DyPs (dye-decolorizing peroxidases) (EC 1.11.1.19) represent a new family of haem peroxidases widespread in bacteria, archaea, fungi and other micro-organisms. In the present study, we expressed A. auricula-judae DyP in E. coli, solved the crystal structure of the recombinant enzyme and several site-directed variants, and used PELE (Protein Energy Landscape Exploration) to describe the binding of its typical substrate RB19. The DyP structure is formed by two domains, each of them including an antiparallel four-stranded large β-sheet and two or three helices resulting in a ferredoxin-like fold (plus two additional β-strands). In spite of the obvious similarity between the two domains, only the C-terminal domain harbours a haem cofactor.

Near the confluence of the two domains, a channel provides access to the haem cofactor that, due to its location in DyPs, connects to the top of the haem. H2O2 will enter through this channel to activate the enzyme, forming compound I. However, direct oxidation of typical DyP substrates, such as RB19 and other bulky dyes, by the activated haem is not possible due to the narrow opening of the channel. A possibility suggested by favourable RB19 docking by PELE is low-turnover oxidation at the DyP haem channel. Since the haem-access channel was also identified as a possible RB19-binding site, the G169L variant was also obtained, whose leucine side chain completely blocks the haem-access channel, as shown in the crystal structure of a variant including the G169L mutation, compared with the WT DyP. However, the disappearance of the low-turnover site in the G169L variant (inset) suggests that this site involves the haem-access channel (although a decrease of the maximal turnover was also observed).

> MATSLNTIDIQGDILVGMHKQKQLFYFFAINDPATFKTHLASDIAPVVASVTQLSNVATQPLVALNIAFSNTGLLALGVTDNLGDSLFANGQAKDATSFKESTSSWVPQFAGTGIHGVIILASDTTDLIDQQVASIESTFGSSISKLSSLSASIRPGNEAGHEMFGFLDLIAQPAINGFNTPLPGQNIVDAGVIITGATNDPITRPSWAVGGSFLAFRQLEQLVPEFNKYLLDNAPAGSGSLQARADLLGARMVGRWKSGAPIDLTPTADDPALGADAQRNNNFTYSHAGFDLGSDQSHCPFSAHIRKTRPRADLGGSLTPPNLSAGANSIMRSGIPYGPEVTSAESASNTTTQERGLAFVAYQAQLSQGFHFLQQTSADNANFPPGKTPATVGLDPIIGQNNGQPRVVNGLLPSNSSASLSIPQFVVSHGGEYFFSPPISAIGGRLSA>MGHHHHHHMQTTSNPRMQVRVSLEKLSLYMRQSPNVLTQDDPRPLPKPKKWADFEIPFKVEAAPTPKSGYIDALTFKFYIAVVNPDRSRQYLKLYKEVKYVNVPVGENTYASVYLSPSSVKRITGVEGGRGKWVKYQGVVVEYNGKIVATYSSERGKMEKWWTIQSPSIVETSYYPLLNKDETPFSVFWYDRYPEIMRPNSQQAASSSVPAPF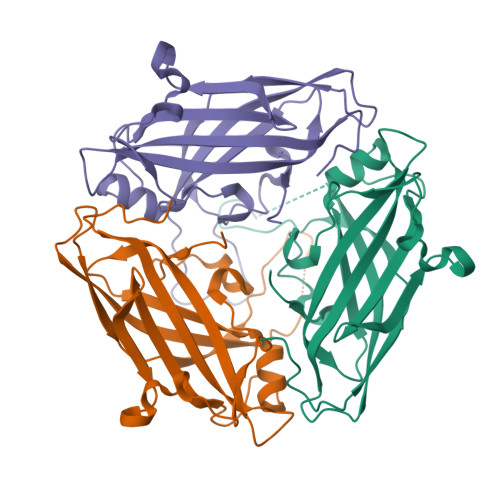GTPVEPPADGELEHHHHHH[3x]> DEPILSFSPKTYSFRQDGRIKEVSVFTYHKKYNPDKHYIYVVRILREGQIEPSFVFRTFDEFQELHNKLSIIFPLWKLPGFPNRMVLGRTHIKDVAAKRKIELNSYLQSLMNASTDVAECDL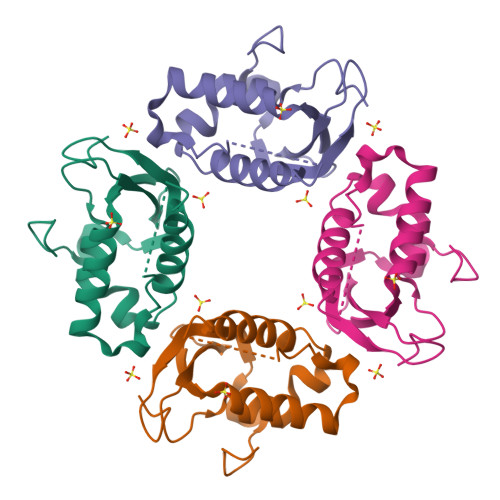VCTFFHPLLRDEKAEGIA>[4x]IVGGRRARPHAWPFMVSLQLRGGHFCGATLIAPNFVMSAAHCVAN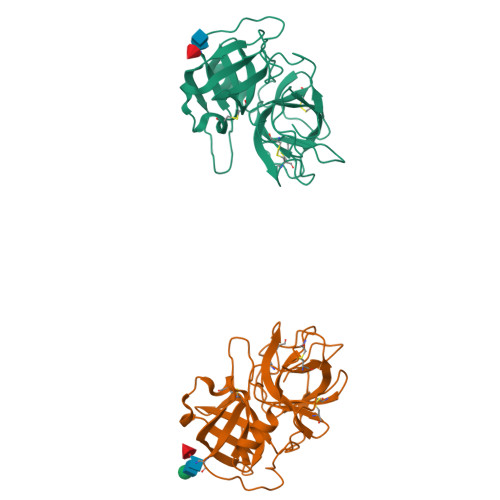VNVRAVRVVLGAHNLSRREPTRQVFAVQRIFENGYDPVNLLNDIVILQLNGSATINANVQVAQLPAQGRRLGNGVQCLAMGWGLLGRNRGIASVLQELNVTVVTSLCRRSNVCTLVRGRQAGVCFGDSGSPLVCNGLIHGIASFVRGGCASGLYPDAFAPVAQFVNWIDSIIQ;>GSTRYVPYTIAVNGTSTPILSKLKISNKQLISYKYLNDKVKSVLKSERGISDLDLKFAKQAKYTVYFKNGKKQVVNLKSDIFTPNLFSAKDIKKIDIDVKQYTKSKKK[2x]>[2x]DFPYDLNALFPE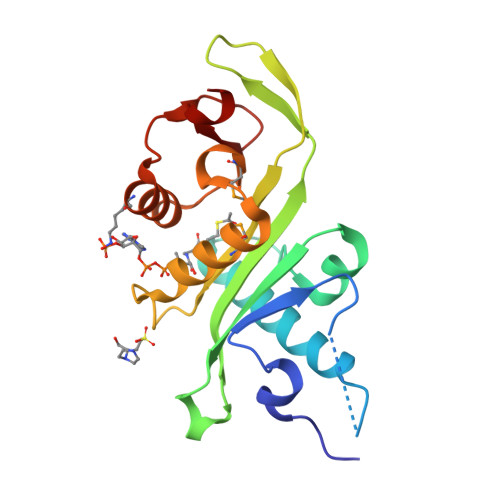RISVLDSNLSAGRKAHGRPDPLPQVTTVIDELGKASSKAQQLPAPITSAAKLQANRHHLYLLKDGEQNGGRGVIVGFLKVGYKKLFLLDQRGAHLETEPLCVLDFYVTETLQRHGYGSELFDFMLKHKQVEPAQMAYDRPSPKFLSFLEKRYDLRNSVPQVNNFVVFAGFFQ> MKAYMFPGQGSQAKGMGRALFDAFPALTARA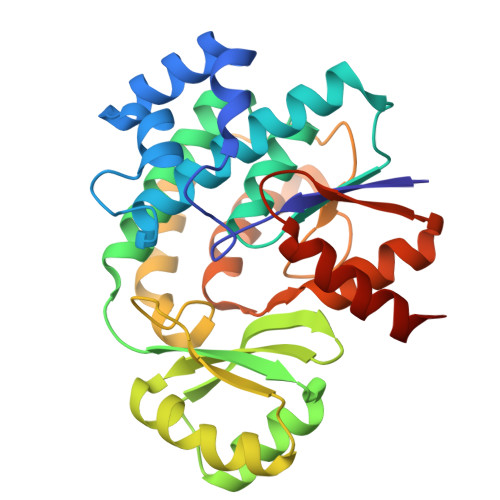DGVLGYSIRALCQDDPDQRLSQTQFTQPALYVVNALSYLKRREEEAPPDFLAGHSLGEFSALFAAGVFDFETGLALVKKRGELMGDARGGGMAAVIGLDEERVRELLDQNGATAVDIANLNSPSQVVISGAKDEIARLQVPFEAAGAKKYTVLRVSAAFHSRFMRPAMVEFGRFLEGYDFAPPKIPVISNVTARPCKADGIRAALSEQIASPVRWCESIRYLMGRGVEEFVECGHGIVLTGLYAQIRRDAQPLVV> MASVHGTTYELLRRQGIDTVFGNPGSNELPFLKDFPEDFRYILALQEACVVGIADGYAQASRKPAFINLHSAAGTGNAMGALSNAWNSHSPLIVTAGQQTRAMIGVEALLTNVDAANLPRPLVKWSYEPASAAEVPHAMSRAIHMASMAPQGPVYLSVPYDDWDKDADPQSHHLFDRHVSSSVRLNDQDLDILVKALNSASNPAIVLGPDVDAANANADCVMLAERLKAPVWVAPSAPRCPFPTRHPCFRGLMPAGIAAISQLLEGHDVVLVIGAPVFRYHQYDPGQYLKPGTRLISVTCDPLEAFRAPMGDAIVADIGAMASALANLVEESSRQLPTAAPEPAKVDQDAGRLHP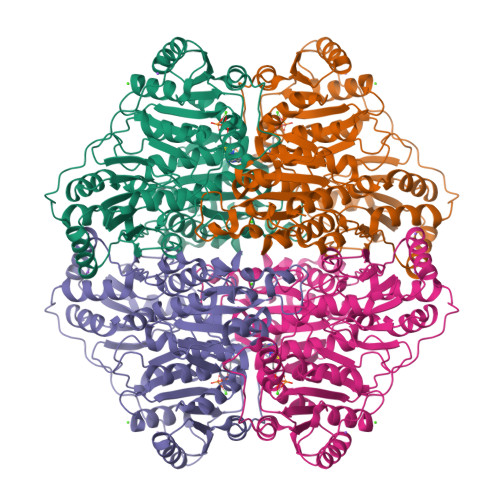ETVFDTLNDMAPENAIYLNESTSTTAQMWQRLNMRNPGSYYFCAAGGLGFALPAAIGVQLAEPERQVIAVIGDGSANYSISALWTAAQYNIPTIFVIMNNGTYGALRWFAGVLEAENVPGLDVPGIDFRALAKGYGVQALKADNLEQLKGSLQEALSAKGPVLIEVSTVSPVKRSHHHHHH methyl 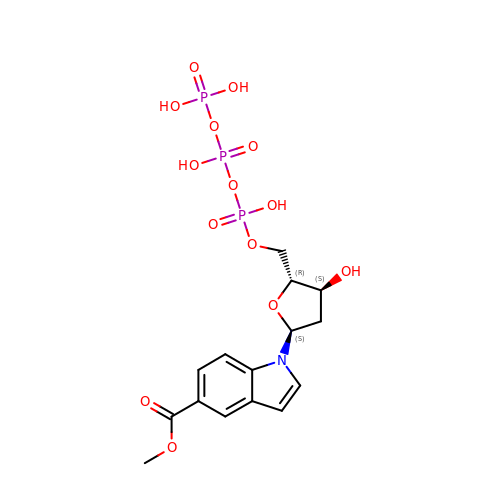1-{2-deoxy-5-O-[(S)-hydroxy{[(S)-hydroxy(phosphonooxy)phosphoryl]oxy}phosphoryl]-alpha-D-erythro-pentofuranosyl}-1H-indole-5-carboxylate | C15 H20 N O14 P3 | QKUDYNPYMMJGEH-MJBXVCDLSA-N>HMLGKVALEEAFALPRHKERTRWWAGLFAIDPDKHAAEINDITEQRIKYMNEHGVGYTILSYTAPGVQDVWDPKEAQALAVEVNDYIADAIKAHPDR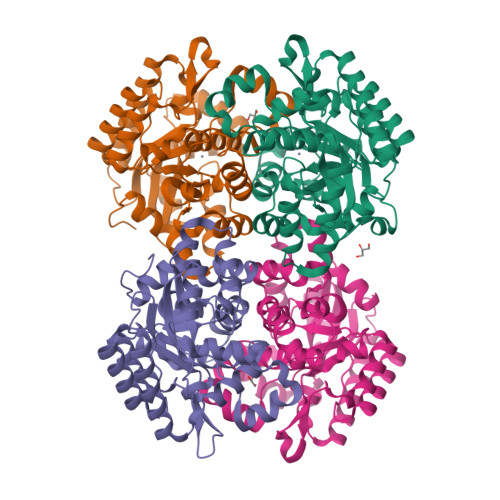LGAFATLSMHDPKEAAEELRRVVTKYGFKGALVNDTQRAGADGDDMIFYDGPEWDVFWSTVTDLDVPFYLHPRNPTGSIHEKLWAKRSWLIGPPLSFAQGVSLHALGMVTNGVFDRHPKLQIVLGHLGEHIPFDMWRINHWFEDIKKPLGLSCKLTIREYFARNLWITTSGHFSTSTLQFCLGEVGADRILFSIDYPFENFSDACTWYDGLAINDVDKRKIGKDNAKKLFKLPQFYQSEDHHHHHH[4x]> ACQCPDAISGWTHTDYQCHGLEKKMYRHVYAICMNGSQVYCR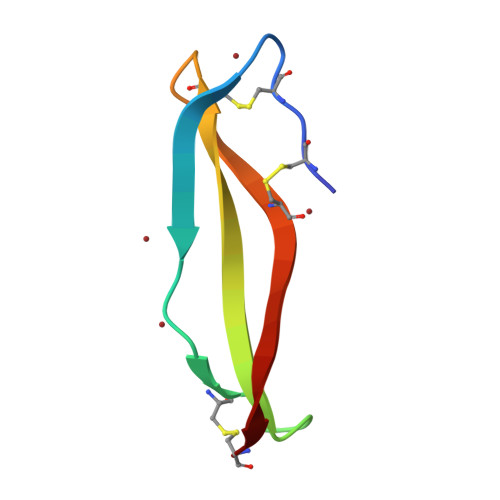TEWGSSC>[8x]MAHHHHHHMVHEATASAPVNIACIKYWGKRDTRLILPTNSSLSVTLDQDHLRSTTTSRADASFEAGDRLWLNGREEAIKEGGRLAVCIKELRAWRKEMETKDKNLPKLSEWPLRIASYN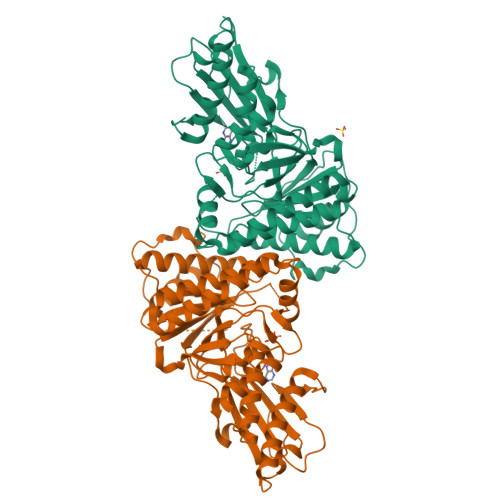NFPTAAGLASSASGLAALVASLASLYSLPQSPSQLSLVARQGSGSACRSLFGGFVAWREGTDPAGSDSLAEEVAPREHWPEMHALICVVSDAKKGTSSTSGMQKTVETSTLLQERLRVVPKRMDAISQAIKARDFAEFAKLTMADSNSFHAVCLDTAPPIFYLNDVSRAIIAVVEELNRAAGEIIAAYTFDAGPNAVIYTLEKNMPFVLGAIKRFFPTSEEFESPFQTGVRDLPEGFNTGVVREGGWEKGAVKGLIHTRVGDGPRVLEKEDSLLGENGVPKVLA> MKKNFFHLLIMLICSYISFAYANISDYRVMTWNLQGSSAST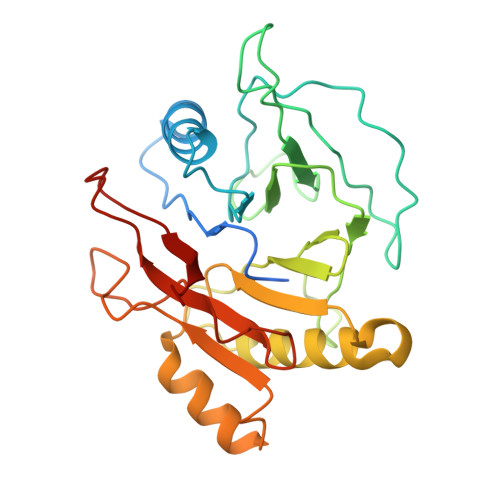ESKWNINVRQLLSGTAGVDILMVQEAGAIPTSAVRTGRHIQPFGVGIPIDEYTWNLGTTRRQDIRYIYYSPIDVGARRVNLAIVTRRRADNVYVLRPTTVASRPIIGIGLGNDVFLTTHALASGGPDAAAIVRVTYNFFRTPQMRHLSWLLGGDFNRAPDRLESDLMTEHLERLVTIIAPTEPTQIGGNILDYGVIVDRAPYSQRVEALRNPQLASDHYPVAFEAQHCG> MKIVSLETHIVAVPPPHVGGMYWIFVKLKTDDGIEGVGEIYSATFGPKAMAPIIDDVFE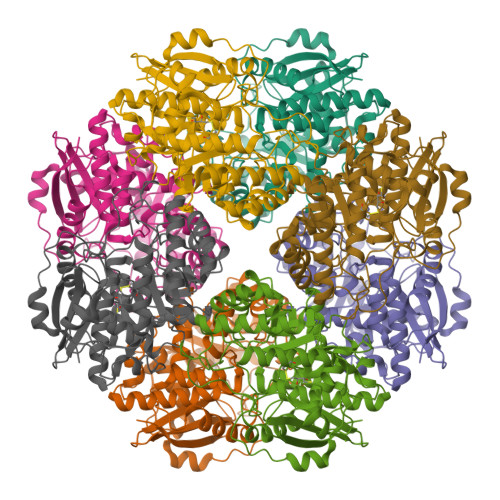RHLLNRDPHHVERLFRQAYSSGFTQRPDLTMMGVVSGLEMACWDIIGKAAAKPVYELLGGRIHERLRSYTYLYPKNAKGEYDYDDPDLAAECAAENVKLGFTAVKFDPAGPYTAYSGHQLSLEVLDRCELFCRRVREAVGSKADLLFGTHGQMVPSSAIRLAKRLEKYDPLWFEEPVPPGQEEAIAQVAKHTSIPIATGERLTTKYEFHKLLQAGGASILQLNVARVGGLLEAKKIATLAEVHYAQIAPHLYNGPVGAAASIQLATCTPNFLIQESIMTWGGFHAEVVKTPIRWEDGYIIPSNEPGLGIELDMDVVKRHTPYTGERLHLQMGEHPVDVKDLAPAKGAENLYFQ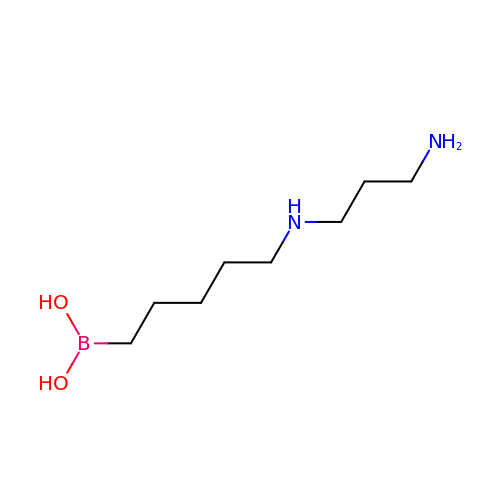{5-[(3-aminopropyl)amino]pentyl}boronic acid | C8 H21 B N2 O2 | WPADTVBHZOIAHR-UHFFFAOYSA-N>EFADAPIDTKTTMDYITPSFANKAGKPKACYVTLVRNKELKGLLSSIKYVENKINKKFPYPWVFLNDEPFTEEFKEAVTKAVSSEVKFGILPKEHW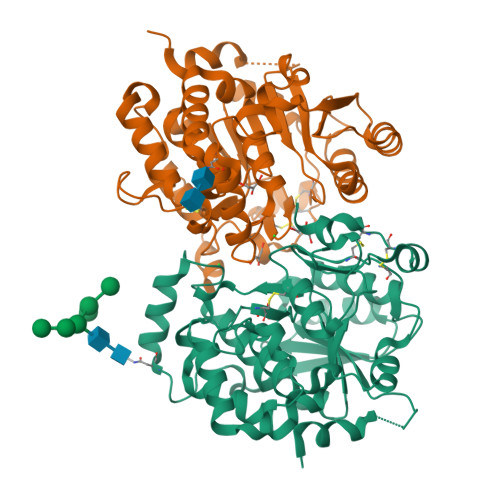SYPEWINQTKAAEIRADAATKYIYGGSESYRHMCRYQSGFFWRHELLEEYDWYWRVEPDIKLYCDINYDVFKWMQENEKVYGFTVSIHEYEVTIPTLWQTSMDFIKKNPEYLDENNLMSFLSNDNGKTYNLCHFWSNFEIANLNLWRSPAYREYFDTLDHQGGFFYERWGDAPVHSIAAALFLPKDKIHYFSDIGYHHPPYDNCPLDKEVYNSNNCECDQGNDFTFQGYSCGKEYYDAQGLVKPKNWKKFRE[2x]> DCPSGWSSYEGNCYKFFQQKMNWADAERFCSEQAKGGHLVSIKIYSKEKDFVGDLVTKNIQS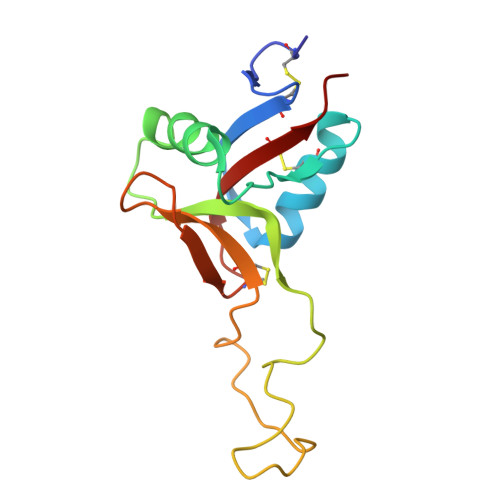SDLYAWIGLRVENKEKQCSSEWSDGSSVSYENVVERTVKKCFALEKDLGFVLWINLYCAQKNPFVCKSPPP>TLNESLQTEKFDFGTMVQWAYDHKYAEESKIAYEYALAAGSDSNARAFLATNSQAKHVKDCATMVRHYLRAETQALSMPAYIKARCKLATGEGSWKSILTFFNYQNIELITFINALKLWLKGIPKKNCLAFIGPPNTGKSMLCNSLIHFLGGSVLSFANHKSHFWLA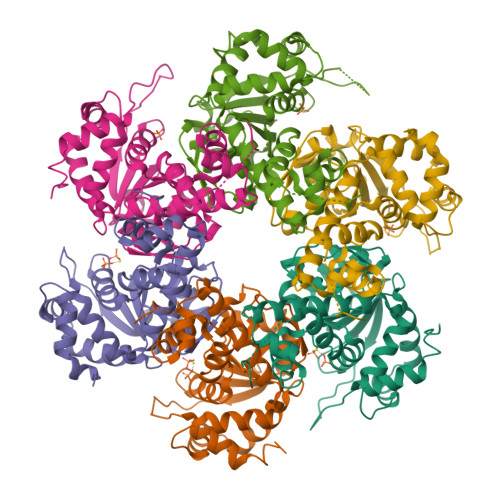SLADTRAALVDDATHACWRYFDTYLRNALDGYPVSIDRKHKAAVQIKAPPLLVTSNIDVQAEDRYLYLHSRVQTFRFEQPCTDESGEQPFNITDADWKSFFVRLWGRLDLIDEEEDSEEDGDSMRTFTCSARNTNAVD[12x]>[2x]MDSISLRVALNDGNFIPVLGFGTTVPEKVAKDEVIKATKIAIDNGFRHFDSA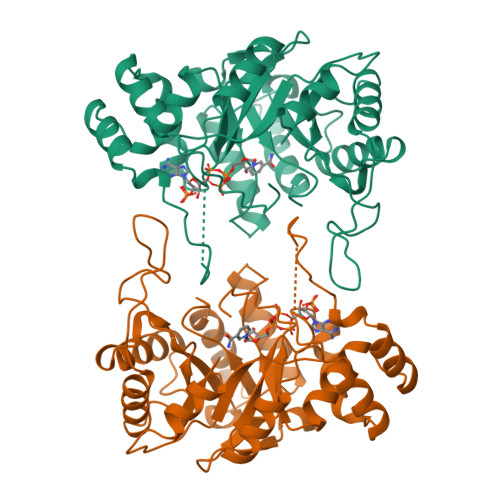YLYEVEEEVGQAIRSKIEDGTVKREDIFYTSKLWSTFHRPELVRTCLEKTLKSTQLDYVDLYIIHFPMALQPGDIFFPRDEHGKLLFETVDICDTWEAMEKCKDAGLAKSIGVSNFNCRQLERILNKPGLKYKPVCNQVECHLYLNQSKMLDYCKSKDIILVSYCTLGSSRDKTWVDQKSPVLLDDPVLCAIAKKYKQTPALVALRYQLQRGVVPLIRSFNAKRIKELTQVFEFQLASEDMKALDGLNRNFRYNNAKYFDDHPNHPFTDE>[9x]MLNYNAPIDGQKSSIDGAGSDQMNTFYWLKKAIIQARKDQYFMPLASVTNMPKNMGKTIKVYEYVPLLDDRNINDQGIDANGAHIVNGNLYGSSKDIGTITSKLPLLTENGGRVNRVGFTRLSREGSIHKFGFFYEFTQESLDFDSDDQLKEHLSRELMNGAVQITEAVLQKDLLAAAGTVLYAGAATSDATITGEGSTPSVITYKNLMRLDAILTDNRTPTQTTIITGSRLVDTKVIGGTRVMYVGSELVPDLKAMKDLFGNKAF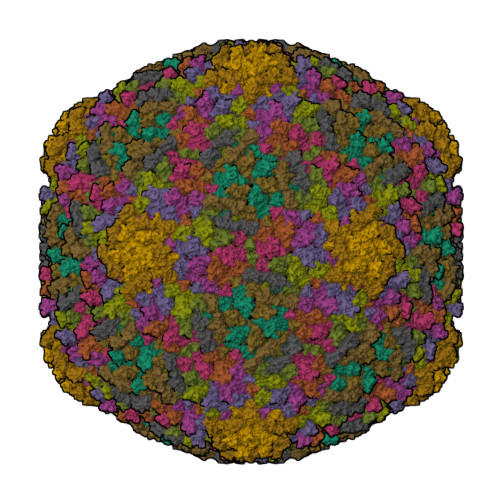IEIQHYGDAGTLMNGEIGTIDKFRIIQVPEMLHWAGAGAAATDANPGYRTSTVNGTEHYDVYPVLVVGDDSFTTIGFQTDGKSVKFNVMTKMPGKETADRNDPYGETGFSSIKWYYGILVKRPERIAVMKAVAPL;>[3x]MPELKVAFNKDTYVATVLDASGSVPSGSVNVGTFFHPDETYPDSYVIYHGVRELLYKRSEVDPAQPGFWPENITNMQAVTIDNKATARLVLNTSLPRVVSTIEGGKVTLSVVALGGKAPLKYKWEFRAPNASTWTAVSGQTTANLVLDNIDADKAGEYKVTVTDAAGTSVDSTALVAVGAYPPPALTGIKATPTSLSLSVATDAAGKTVALSAIPTDAELGTLSIKTAPDSARATATISGSTLTVKPVAAGAATSVVVTNGKVDVTITINVAA> KRRMPTDI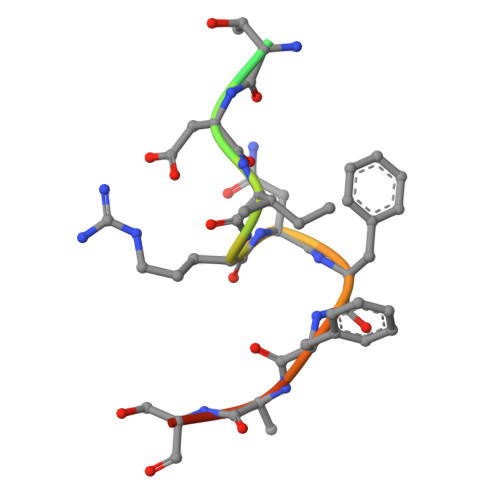RNFFHSKR> GSMEWKLFADLAEVAGSRTVRVDVDGDATVGDALDALVGAHPALESRVFGDDGELYDHINVLRNGEAAALGEATAAGDELALFPP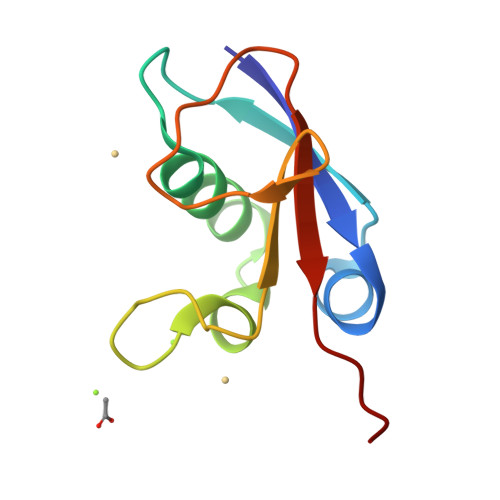VSGG> NVAAAERQLRELESTFDGRLGFVALDTATGARIAHRGDERFPFCSTSKMMLCAAVLARSAGEPALLQRRIAYAKGDLIRYSPITEQHVGAGMSVAELCAATLQYSDNTAANLLIALLGGPQTVTAYARSIGDATFRLDRREPELNTALPGDERDTTTPAAMAASVHRLLVGDALGAAQRAQLN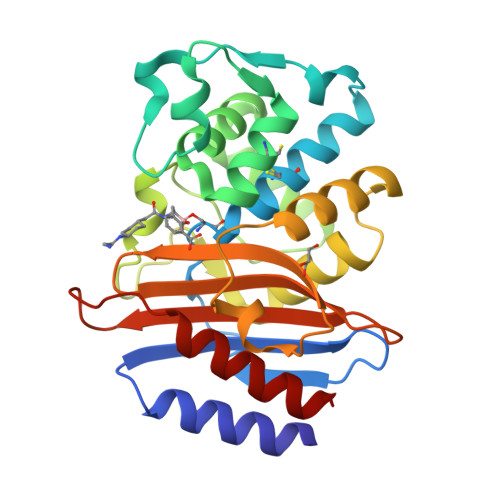AWMLGNKTGDARIRAGVPADWRVADKTGTGDYGTANDIGVAYPPNRAPIVFIVYTTMRNPNAQARDDVIASATRIAARAFA>MDKCKKVYENYPVSKCQLANQCNYDCKLKKHARSGECFYDEKRNLQCICDYCEY[7x];> 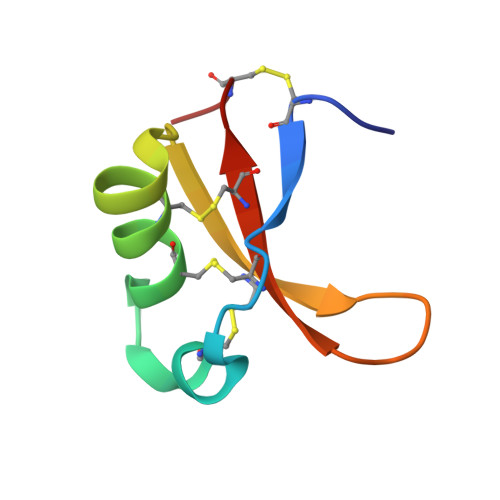MDKCKKVYENYPVSKCQLANQCNYDCKLDKHARSGECFYDEKRNLQCICDYCEY>MPREYEFAEKILFTEEEIRTRIKEVAKRIADDYKGKGLRPYVNPLVLISVLKGSFMFTADLCRALCDFNVPVRMEFICVSSYGEGLTSSGQVRMLLDTRHSIEGHHVLIVEDIVNTALTLNYLYHMYFTRRPASLKTVVLLDKREGRRVPFSADYVVANIPNAFVIGYGLDYDDTYRELRDIVVLRPEVYAER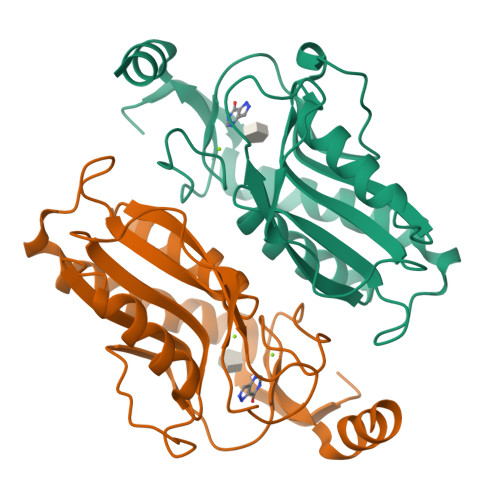EAARGKKQRAIGSADTDRDAKREFHSKY[2x]> SITDILSAEDIAAALQECQDPDTFEPQKFFQTSGLSKMSASQVKDIFRFIDNDQSGYLDGDELKYFLQKFQSDARELTESETKSLMDAADNDGD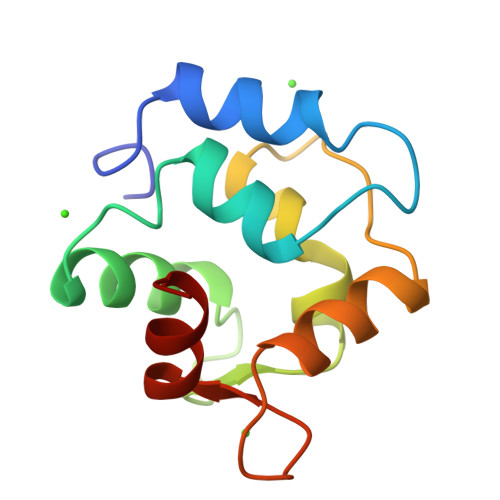GKIGADEFQEMVHS>[5x]MYSTAVLLNKISPTRDGQTMTLADLQYLSFSELRKIFDDQLSWGEARHLYHETIEQKKNNRLLEARIFTRANPQLSGAIRLGIERDSVSRSYDEMFGARSSSFVKPGSVASMFSPAGYLTELYREAKDLHFSSSAYHLDNRRPDLADLTLSQSNMDTEISTLTLSNELLLEHITRKTGGDSDALMESLSTYRQAIDTPYHQPYETIRQVIMTHDSTLSALSRNPEVMGQAEGASLLAILANISPELYNILTEEITEKNADALFAQNFSENITPENFASQSWIAKYYGLELSEVQKYLGMLQNGYSDSTSAYVDNISTGLVVNNESKLEAYKITRVKTDDYDKNINYFDLMYEGNNQFFIRANFKVSREFGATLRKNAGPSGIVGSLSGPLIANTNFKSNYLSNISDSEYKNGVKIYAYRYTSSTSATNQGGGIFTFESYPLTIFALKLNKAIRLCLTSGLSPNELQTIVRSDNAQGIINDSVLTKVFYTLFYSHRYALSFDDAQVLNGSVINQYADDDSVSHFNRLFNTPPLKGKIFEADGNTVSIDPDEEQSTFARSALMRGLGVNSGELYQLGKLAGVLDAQNTITLSVFVISSLYRLTLLARVHQLTVNELCMLYGLSPFNGKTTASLSSGELPRLVIWLYQVTQWLTEAEITTEAIWLLCTPEFSGNISPEISNLLNNLRPSISEDMAQSHNRELQAEILAPFIAATLHLASPDMARYILLWTDNLRPGGLDIAGFMTLVLKESLNANETTQLVQFCHVMAQLSLSVQTLRLSEAELSVLVISGFAVLGAKNQPAGQHNIDTLFSLYRFHQWINGLGNPGSDTLDMLRQQTLTADRLASVMGLDISMVTQAMVSAGVNQLQCWQDINTVLQWIDVASALHTMPSVIRTLVNIRYVTALNKAESNLPSWDEWQTLAENMEAGLSTQQAQTLADYTAERLSSVLCNWFLANIQPEGVSLHSRDDLYSYFLIDNQVSSAIKTTRLAEAIAGIQLYINRALNRIEPNARADVSTRQFFTDWTVNNRYSTWGGVSRLVYYPENYIDPTQRIGQTRMMDELLENISQSKLSRDTVEDAFKTYLTRFETVADLKVVSAYHDNVNSNTGLTWFVGQTRENLPEYYWRNVDISRMQAGELAANAWKEWTKIDTAVNPYKDAIRPVIFRERLHLIWVEKEEVAKNGTDPVETYDRFTLKLAFLRHDGSWSAPWSYDITTQVEAVTDKKPDTERLALAASGFQGEDTLLVFVYKTGKSYSDFGGSNKNVAGMTIYGDGSFKKMENTALSRYSQLKNTFDIIHTQGNDLVRKASYRFAQDFEVPASLNMGSAIGDDSLTVMENGNIPQITSKYSSDNLAITLHNAAFTVRYDGSGNVIRNKQISAMKLTGVDGKSQYGNAFIIANTVKHYGGYSDLGGPITVYNKTKNYIASVQGHLMNADYTRRLILTPVENNYYARLFEFPFSPNTILNTVFTVGSNKTSDFKKCSYAVDGNNSQGFQIFSSYQSSGWLDIDTGINNTDIKITVMAGSKTHTFTASDHIASLPANSFDAMPYTFKPLEIDASSLAFTNNIAPLDIVFETKAKDGRVLGKIKQTLSVKRVNYNPEDILFLRETHSGAQYMQLGVYRIRLNTLLASQLVSRANTGIDTILTMETQRLPEPPLGEGFYATFVIPPYNLSTHGDERWFKLYIKHVVDNNSHIIYSGQLTDTNINITLFIPLDDVPLNQDYHAKVYMTFKKSPSDGTWWGPHFVRDDKGIVTINPKSILTHFESVNVLNNYSAPMDFNSASALYYWELFYYTPMMCFQRLLQEKQFDEATQWINYVYNPAGYIVNGEIAPWIWNCRPLEETTSWNANPLDAIDPDAVAQNDPMHYKIATFMRLLDQLILRGDMAYRELTRDALNEAKMWYVRTLELLGDEPEDYGSQQWAAPSLSGAASQTVQAAYQQDLTMLGRGGVSKNLRTANSLVGLFLPEYNPALTDYWQTLRLRLFNLRHNLSIDGQPLSLAIYAEPTDPKALLTSMVQASQGGSAVLPGTLSLYRFPVMLERTRNLVAQLTQFGTSLLSMAEHDDADELTTLLLQQGMELATQSIRIQQRTVDEVDADIAVLAESRRSAQNRLEKYQQLYDEDINHGEQRAMSLLDAAAGQSLAGQVLSIAEGVADLVPNVFGLACGGSRWGAALRASASVMSLSATASQYSADKISRSEAYRRRRQEWEIQRDNADGEVKQMDAQLESLKIRREAAQMQVEYQETQQAHTQAQLELLQRKFTNKALYSWMRGKLSAIYYQFFDLTQSFCLMAQEALRRELTDNGVTFIRGGAWNGTTAGLMAGETLLLNLAEMEKVWLERDERALEVTRTVSLAQFYQALSSDNFNLTEKLTQFLREGKGNVGASGNELKLSNRQIEASVRLSDLKIFSDYPESLGNTRQLKQVSVTLPALVGPYEDIRAVLNYGGSIVMPRGCSAIALSHGVNDSGQFMLDFNDSRYLPFEGISVNDSGSLTLSFPDATDRQKALLESLSDIILHIRYTIRSENLYFQGDYKDDDDKLEHHHHHH

ABC toxin complexes (Tcs) are a class of α-pore forming toxins (αPFTs) that consist of three subunits capable of assembling into a single protein apparatus with the ability to shuttle and translocate toxic peptides into target cells. The two TcAs termed Xn-XptA1 and Xn-XptA2 are the targeting components of each complex and display variations in insect specificity. The TcAs are the largest subunits of the complex and contain a translocation channel with hydrophobic loops at the end allowing for membrane permeation. Upon TcA binding and an environmental pH change, the complex undergoes a conformational change into an active state in which the translocation channel is exposed and pierces the target cell membrane.

The second strategy we implemented to alter the host tropism of Xn-XptA2 was to substitute a full RBD from the homologous TcA Photorhabdus luminescens TcdA1 (Pl-TcdA1) into Xn-XptA2. Regarding the domain substitution, we decided to substitute the Xn-XptA2 RBD C (F1659-G1787) for the analogous RBD D (A1643-N1752) in Pl-TcdA1 due to these RBDs being closest to the membrane before pore formation. This was achieved by excising the sequence of DNA encoding the TcdA1 RBD D and ligating this sequence into the scaffold sequence encoding for Xn-XptA2 after excision of the homologous RBD C sequence. High-resolution structure determination of the Xn-XptA2 RBD C chimera was achieved through cryo-EM single particle analysis, yielding a final high-resolution structure at 3.6 Å resolution. Structural analysis displayed a stable chimera in the State 1 conformation, indicating that the full RBD substitution did not have an allosteric effect on alternative domains. Upon further inspection, the Pl-TcdA1 RBD D within the Xn-XptA2 scaffold was mostly identical in structure to Pl-TcdA1 wt RBD D, with all β-sheets being conserved and the loss of one α-helix at position N1651-G1656. When the Panc1 and MiaPaCa2 cells were exposed to the Xn-XptA2 RBD C chimera Tc, we observed no significant difference in cell viability for both cell lines. Due to the structural integrity of Pl-TcdA1 RBD D within the Xn-XptA2 RBD C chimera, we conclude that RBD C is not responsible for host tropism to Panc1 and MiaPaCa2 cells through the process of elimination. Furthermore, we display the capability to substitute alternative RBDs into the Xn-XptA2 scaffold while maintaining structural stability.> SASGVRIDPTQTQNLGVKTATVTRGPLTFAQSFPANVSYNEYQYAIVQARAAGFIDKVYPLTVGDKVQKGTPLLDLTIPDWVEAQSEYLLLRETGGTATQTEGILERLRLAGMPEADIRRLIATQKIQTRFTLKAPIDGVITAFDLRAGMNIAKDNVVAKIQGMDPVWVTAAIPESIAWLVKDASQFTLTVPARPDKTLTIRKWTLL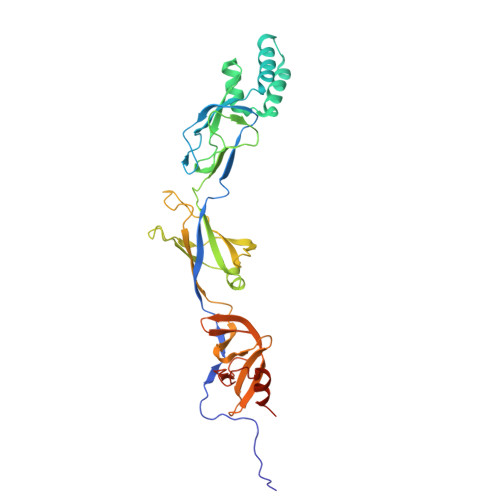PGVDAATRTLQLRLEVDNADEALKPGMNAWLQLNTASEPMLLIPSQALIDTGSEQRVITVDADGRFVPKRVAVFQASQGVTALRSGLAEGEKVVSSGLFLIDSEANISGALERMRSESATHAHHHHHHH>[2x]MMFLRQEDFATVVRSTPLVSLDFIVENSRGEFLLGKRTNRPAQGYWF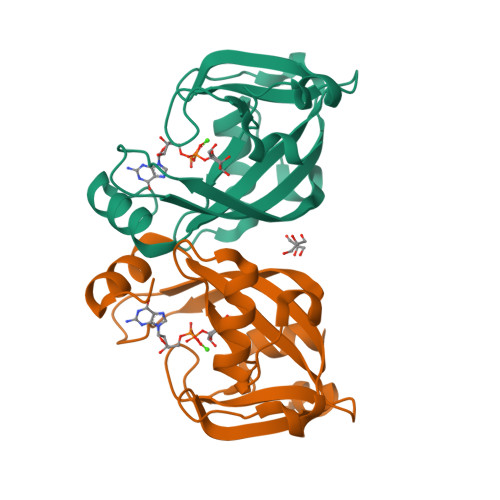VPGGRVQKDETLEAAFERLTMAELGLRLPITAGQFYGVWQHFYDDNFSGTDFTTHYVVLGFRFRVAEEELLLPDEQHDDYRWLTPDALLASENVHANSRVYFNNDPRAIIGLNKKEVKNV> MGSSHHHHHHSQDPNSMPDNTIQWDKDADGIVTLTMDDPSGSTNVMNEAYIESMGKAVDRLVAEKDSITGVVVASAKKTFFAGGDVKTMIQARPEDAGDVFNTVETIKRQLRTLETLGKPVVAAINGAALGGGLEIALACHHRIAADVKGSQLGLPEVTLGLLPGGGGVTRTVRMFGIQNAFVSVLAQGTRFKPAKAKEIGLVDELVATVEELVPAAKAWIKEELKANPDGAGVQPWDKKGYKMPGGTPSSPGLAAILPSFPSNLRKQLKGAPMPAPRAILAAAVEGAQVDFDTASRIESRYFASLVTGQVAKNMMQAFFFDLQAINAGGSRPEGIGKTPIKRIGVLGAGMMGAGIAYVSAKAGYEVVLKDVSLEAAAKGKGYSEKLEAKALERGRTTQERSDALLARITPTADAADFKGVDFVIEAVFENQELKHKVFGEIEDIVEPNAILGSNTSTLPITGLATGVKRQEDFIGIAFFSPVDKMPLVEIIKGEKTSDEALARVFDYTLAIGKTPIVVNDSRGFFTSRVIGTFVNEALAMLGEGVEPASIEQAGSQAGYPAPPLQLSDELNLELMHKIAVATRKGVEDAGGTYQPHPAEAVVEKMIELGRSGRLKGAGFYEYADGKRSGLWPGLRETFKSGSSQPPLQDMIDRMLFAEALETQKCLDEGVLTSTADANIGSIMGIGFPPWTGGSAQFIVGYSGPAGTGKAAFVARARELAAAY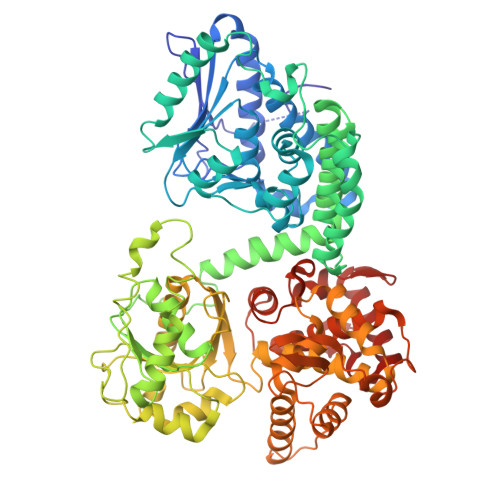GDRFLPPESLLS> SGGNAEEITEKATLVGIEAWLLAKDEEQKKKVRTLNRQVKKLLQQNDLDQAKRVLDQLKSVLEDLKS;> MAHHHHHHMLPIQKKVGYLIKDDSEKQAT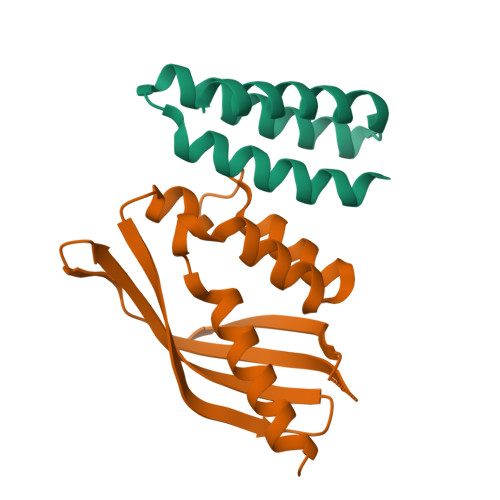ITNTKYSTLANPYISVANIMLQNYVKQREKYNYDTLKEQFTFIKNASTSIVYMQFANFMNIDNSLSPVIRYQKLYRRSINIISINNINNNEATVTFESLAQNNTGEILENMLWEAKIGFIMDSISTSTLHNMPFHFIVTSYKLKLLRNKNQQ>MSQFKNIIVTGGAGFIGSNFVHYVYNNHPDVHVTVL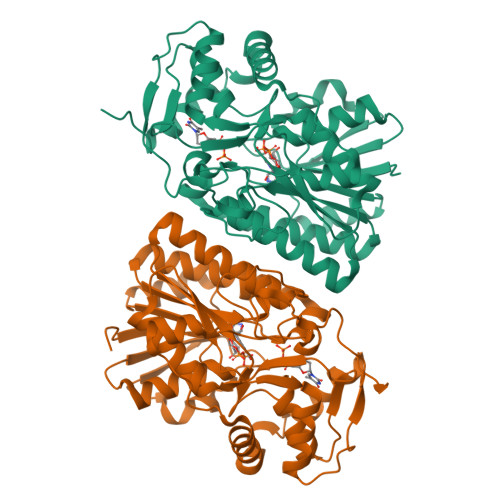DKLTYAGNKANLEAILGDRVELVVGDIADAELVDKLAAKADAIVHYAAESHNDNSLNDPSPFIHTNFIGTYTLLEAARKYDIRFHHVSTDEVYGDLPLREDLPGHGEGPGEKFTAETNYNPSSPYSSTKAASDLIVKAWVRSFGVKATISNCSNNYGPYQHIEKFIPRQITNILAGIKPKLYGEGKNVRDWIHTNDHSTGVWAILTKGRMGETYLIGADGEKNNKEVLELILEKMGQPKDAYDHVTDRAGHDLRYAIDASKLRDELGWTPQFTDFSEGLEETIQWYTDNQDWWKAEKEAVEANYAKTQEVIK[2x]>[4x]CAGA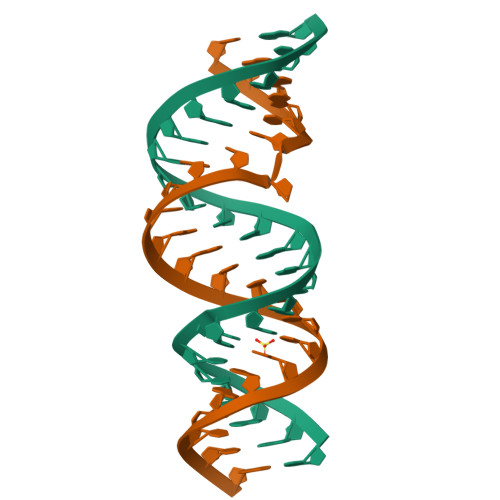CUGCGAGGGCCCUCGAGUUUG>MKPHPWFFGKIPRAKAEEMLSKQRHDGAFLIRESESAPGDFSLSVKFGNDVQHFKVLRDGAGK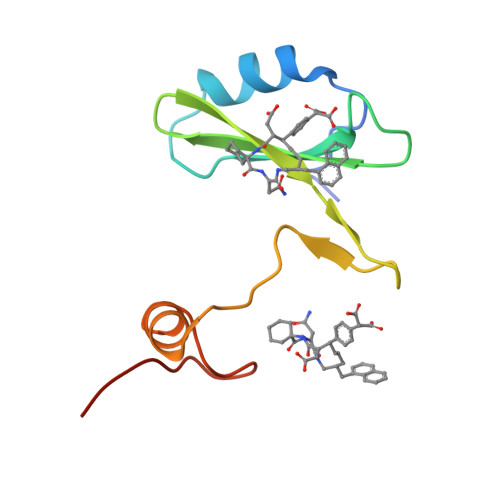YFLWVVKFNSLNELVDYHRSTSVSRNQQIFLRDIEQ[2x]>[2x]HGHSSSDPVYPCGICTNEVNDDQDAILCEASCQKWFHRICTGMTETAYGL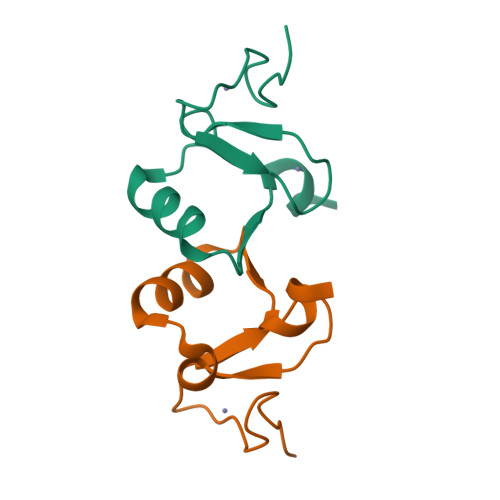LTAEASAVWGCDTCMAD>GSSHHHHHHSSGLVPRGSHMKSTSVSPFHLPLNHPTYLIWSANTSLGKTLVSTGIAASFLLQQPSSSATKLLYLKPIQTGFPSDSDSRFVFSKLDSLSLRRQIPISISNSVLHSSLPAAKSLGLNVEVSESGMCSLNFRDEKTVTGAPELLCKTLYAWEAAISPHLAAERENATVEDSVVLQMIEKCLKEEMECGVKSEKSDLLCLVETAGGVASPGPSGTLQCDLYRPFRLPGILVGDGRLGGISGTIAAYESLKLRGYDIAAVVFEDHGLVNEVPLTSYLRNKVPVLVLPPVPKDPSDDLIEWFVESDGVFKALKETMVLANLERLERLNGMAKLAGEVFWWPFTQHKLVHQETVTVIDSRCGENFSIYKASDNSSLSQQFDACASWWTQGPDPTFQAELAREMGYTAARFGHVMFPENVYEPALKCAELLLDGVGKGWASRVYFSDNGSTAIEIALKMAFRKFCVDHNFCEATEEEKHIVVKVIALRGSYHGDTLGAMEAQAPSPYTGFLQQPWYTGRGLFLDPPTVFLSNGSWNISLPESFSEIAPEYGTFTSRDEIFDKSRDASTLARIYSAYLSKHLQEHSGVRQSAHVGALIIEPVIHGAGGMHMVDPLFQRVLVNECRNRKIPVIFDEVFTGFWRLGVETTTELL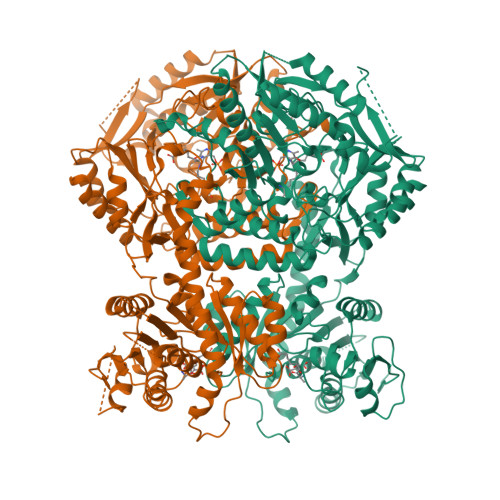GCKPDIACFAKLLTGGMVPLAVTLATDAVFDSFSGDSKLKALLHGHSYSAHAMGCATAAKAIQWFKDPETNHNITSQGKTLRELWDEELVQQISSHSAVQRVVVIGTLFALELKADASNSGYASLYAKSLLIMLREDGIFTRPLGNVIYLMCGPCTSPEICRRLLTKLYKRLGEFNRT[2x]> MPKTISVRVT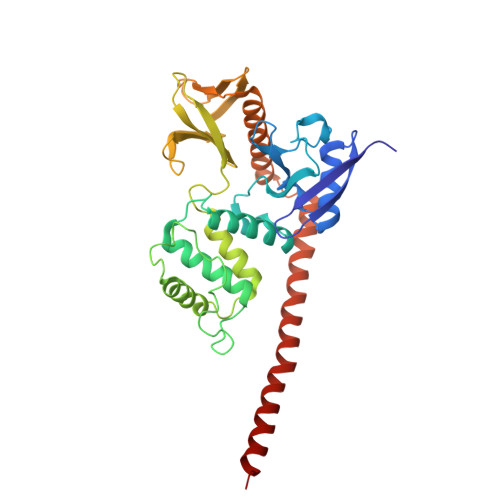TMDAELEFAIQPNTTGKQLFDQVVKTIGLREVWFFGLQYQDTKGFSTWLKLNKKVTAQDVRKESPLLFKFRAKFYPEDVSEELIQDITQRLFFLQVKEGILNDDIYCPPETAVLLASYAVQSKYGDFNKEVHKSGYLAGDKLLPQRVLEQHKLNKDQWEERIQVWHEEHRGMLREDAVLEYLKIAQDLEMYGVNYFSIKNKKGSELWLGVDALGLNIYEQNDRLTPKIGFPWSEIRNISFNDKKFVIKPIDKKAPDFVFYAPRLRINKRILALCMGNHELYMRRRKPDTIEVQQMKAQAREEKHQKQMERAMLENEKKKREMAEKEKEKIEREKEE>[8x]MGSSHHHHHHSSGLVPRGSMNIFDVKDKYILITGASSGLGHHIAELFAKEGANIVICARRLERLKELESHIKNEYGVQVYTFALDVNDRSAVKDMLSSLEAEGVTIDVLINNAGVSDTKRFLDYNDEDWDKIVDTNLKAPWQCAQEVVQHMIKAERKGSIINITSILSQSTNLGVSPYCASKAGLRHLTEVMAVELARFGINVNAIAPGYMITEINEEYLTSEVGQQLLKKIPTRKFVEFDDLNGPLLLLASQAGQGITGIEIKVDGGHSAAPI

Here, we describe the 2.4 Å resolution crystal structure determined for SDR-WM99c, one of a pair of hypothetical proteins also encoded within this island. Its structure displays a tertiary fold attributable to a short-chain dehydrogenase (SDR) of classical architecture. The relatively large SDR family catalyses a broad range of reactions utilizing NAD(P)-dinucleotide cofactors. This robust enzyme fold is known to accommodate a wide variety of substrates and thus yields metabolic functions spanning several EC classes from oxidoreductases and lyases to isomerases.

The enzyme crystallized in the apo form, with no cofactor or substrate bound in any subunit. All eight chains can be completely traced from residues 2 to 254 (a total chain length of 255 residues). All eight chains align closely, with an r.m.s.d. of 0.3–0.5 Å (Cα atoms). In solution, the native mass determined for SDR-WM99c was consistent with a stable tetramer, and no dimeric population was evident in elution traces. The αβα core is extended in the case of SDR-WM99c by a capping helix–turn–helix feature (helices α′ and α′′; Asn197–Ile213). Helices α′ and α′′ display relatively high B factors (ranging from 146 to 203 Å2), indicating dynamic mobility in this region. Overlay of SDR-WM99c and its closely related SDR structures immediately reveals retention of the geometry of side chains for this catalytic tetrad. These four active-site residues are thereby identified in SDR-WM99c as Asn117 (α4), Ser146 (β5–α6 loop), Tyr159 (α5) and Lys163 (α5). No density consistent with either cofactor or substrate was evident within this structure of SDR-WM99c; however, overlay with the structure of the related FabG1–NADP complex clearly reveals the cofactor site. By direct analogy, in SDR-WM99c the adenine ring and the ribose phosphate are proposed to engage α4 helix residues (Asp66 and Val67) and β1–α1 loop residues (Thr14, Gly15 and Ser17), respectively. In SDR-WM99c, such a cleft appears to be located between helices α′ and α′′, i.e. in a markedly flexible region of the apoenzyme structure.> PAKDVQICPIAVDTTVFRSRTWDRLKFEIEYGLQRGTTANSYLISADKIALFDPPGESFTDNFVGTLIQRLDLNSLDYVILGHVNANRAHTLKLLLSLAPQATIICSNPAAQNLEKLLADAEVNNPIQVMKGNDHL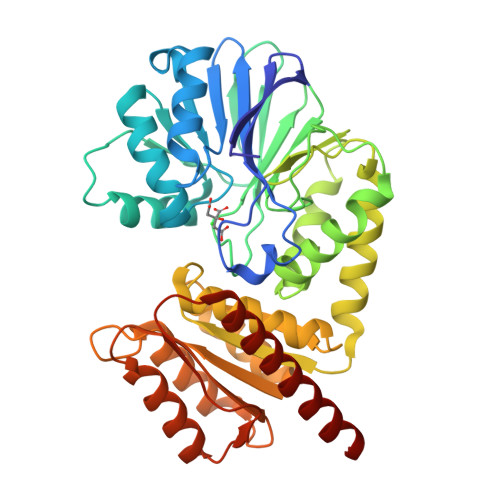DLGRGHELTFIPTPSPRYPGQLCTYDPRTEILFTDKLFGAHVCGDQVFDEGWTIYQEDRRYYFDCLLAPAAAQVSAALNKLEAYPAQTYAPSHGPLVRYGLRELTRNYQQWLSEQQAQALNVALIYASAYGNTSTLAQAIARGITKAGVAVTAINAETSNAEEIKEAIGKSAGFIFGSPTLGGHAPTPIQTALGITLANASKTQLCGVFGSFGWSGEAIDMLENKFRDAGFSFGFDTIRVKFKPTDQTLKMCEEAGTDFAQALKKAEKRR> METRSDVFEFEFSETPLLPCYNIQVSVAQGPRNWLLLSDVLKKLKMSSRIFRCNFPNVEIVTIAEAEFYRQVSASLLFSCSKDLEAFNPESKELLDLVEFTNEIQTLLGSSVEW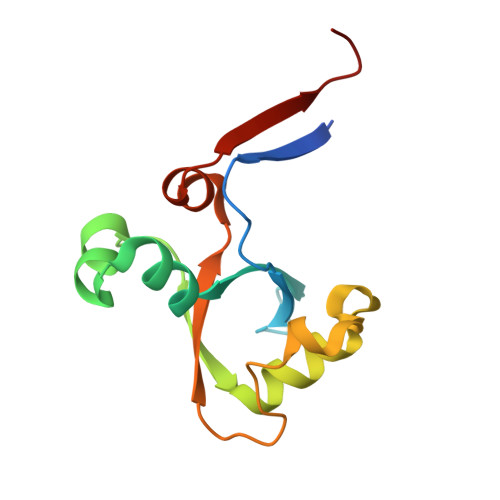LHPSD> MHHHHHHHDGTENPIHDRTSDYHKYLKVKQGDSDLFKLTVSDKRYIWYNPDPKERDSYECGEIVSETSDSFTFKTVDGQDRQVKKDDANQRNPIKFDGVEDMSELSYLNEPAVFHNLRVRYNQDLIYTYSGLFLVAVNPFKRIPIYTQEMVDIFKGRRRNEVAPHIFAISDVAYRSMLDDRQNQSLLITGESGAGKTENTKKVIQYLASVAGRNQANGSGVLEQQILQANPILEAFGNAKTTRNNNSSRFGKFIEIQFNSAGFISGASIQSYLLEKSRVVFQSETERNYHIFYQLLAGATAEEKKALHLAGPESFNYLNQSGCVDIKGVSDSEEFKITRQAMDIVGFSQEEQMSIFKIIAGILHLGNIKFEKGAGEGAVLKDKTALNAASTVFGVNPSVLEKALMEPRILAGRDLVAQHLNVEKSSSSRDALVKALYGRLFLWLVKKINNVLCQERKAYFIGVLDISGFEIFKVNSFEQLCINYTNEKLQQFFNHHMFKLEQEEYLKEKINWTFIDFGLDSQATIDLIDGRQPPGILALLDEQSVFPNATDNTLITKLHSHFSKKNAKYEEPRFSKTEFGVTHYAGQVMYEIQDWLEKNKDPLQQDLELCFKDSSDNVVTKLFNDPNIASRAKKGANFITVAAQYKEQLASLMATLETTNPHFVRCIIPNNKQLPAKLEDKVVLDQLRCNGVLEGIRITRKGFPNRIIYADFVKRYYLLAPNVPRDAEDSQKATDAVLKHLNIDPEQYRFGITKIFFRAGQLARIEEAREQRLESNE

Myosin is a ubiquitously expressed adenosine triphosphate (ATP)-driven motor protein, producing force and directed motion along cytoskeletal actin filament tracks by converting chemical energy from ATP hydrolysis into mechanical work. Despite their specialized cellular functions, all members of the myosin superfamily share a common multistep mechanism of force generation—the chemomechanical actomyosin motor cycle. The myosin motor is thus subject to substantial conformational changes along that cycle, traversing through different actin-attached and –detached states, eventually amplifying them to a large scale rotation of the converter domain and swinging of the adjacent lever arm in the force-generating power stroke. ADP release is key for the regulation of the mechanical motor function of myosin as it controls the fraction of time the motor stays attached to the actin filament.

In a series of crystallization trials using the myosin-II inhibitor blebbistatin, we obtained a previously unknown conformation of myosin in the presence of ADP. We solved the crystal structure of the Dd myosin-II motor domain in complex with blebbistatin and ADP to a resolution of 2.58 Å (see Table 1 for data statistics). The hallmarks of the unique structure are a converter position close to the rigor down position, rearrangements of the active site switches closer together, and a large shift of the P-loop together with the bound ADP towards the protein surface, while the β-phosphate of ADP lost most of its coordination with protein residues. The positions of the active site switches (closed with the P-loop shifted towards the surface), and the converter/lever arm (near down position), as well as the status of the actin-binding cleft (almost closed), the relay helix (straight), and the transducer (almost fully twisted) suggest that the structure resembles a myosin conformation towards the end of the power stroke that promotes ADP release. Blebbistatin was found in the same binding site as observed in the crystal structure of the myosin-II pre-power stroke state, and interacts with residues of the relay and W-helices, as well as active site switches in close proximity to β-strands 5 to 7 of the transducer. Consistently, the converter is rotated by approximately 55° as compared to the up position in the pre-power stroke state, and would need to undergo only a minor 4° to 5° converter rotation to transition to the down position in the rigor state. Similarly, a transition by approximately 1 Å of both the inner and outer actin-binding cleft (myosin-II·ADP·blebbistatin complex: inner cleft: 11.7 Å and outer cleft: 11.3 Å) separates the blebbistatin-bound myosin-II·ADP from the fully closed actin-binding cleft as seen in the apo rigor state, indicating a new actin interface.> MDLVKDVKRELSFSELKGKRVSIDGYNALYQFLAAIRQPDGTPLMDSQGRVTSHLSGLFYRTINILEEGVIPIYVFDGKPPEQKSEELERRRKAKEEAERKLERAKSEGKIEELRKYSQAILRLSNIMVEESKKLLRAMGIPIVQAPSEGEAEAAYLNKLGLSWAAASQDYDAILFGAKRLVRNLTITGKRKLPNKDVYVEIKPELIETEILLKKLGITREQLIDIGIL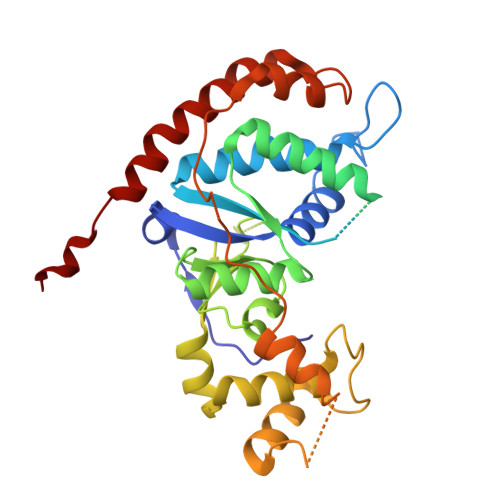IGTDYNPDGIRGIGPERALKIIKKYGKIEKAMEYGEISKKDINFNIDEIRGLFLNPQVVKPEEALDLNEPNGEDIINILVYEHNFSEERVKNGIERLTKAIKEAKGASRQTGLDRWF>[2x]MGRIKNKQFAVIGLGKFGGSICKELHRMGHEVLAVDINEEKVNAYASYATHAVIANATEENELLSLGIRNFEYVIVAIGANIQASTLTTLLLKELDIPNIWVKAQNYYHHKVLEKIGADRIIHPEKDMGVKIAQSLSDENVLNYIDLSDEYSIVELLATRKLDSKSIIDLNVRAKYGCTILAIKHHGDICLSPAPEDIIREQDCLVIMGHKKDIKRFENEGM

KtrAB is a cation channel with a nucleotide-dependent RCK domain. The structure of the KtrAB complex revealed a homodimeric membrane protein (KtrB) assembled with a cytosolic RCK octameric ring, formed by the KtrA protein. KtrA binds nucleotides, ATP or ADP. ATP binding induces the adoption of a square-conformation by the octameric ring and increased K+ flux activity through KtrAB; ADP binding results in a non-square conformation and decreased flux.

The structures of R16K (at 2.7 Å resolution) and R16A (at 3.4 Å resolution) with ATP are very similar to that of the previously determined wild-type KtrA-ATP (WT-ATP), adopting the square conformation. In the ATP-bound rings, these distances are similar in the R16K (30.8/30.8 Å), R16A (29.9/29.9 Å) mutants and wild-type (30.0/30.0 Å) structures. A clue for the role of E125 is revealed by the 2.7 Å structure of the ATP-bound R16K KtrA mutant. In this structure, there was a distinct additional electron-density in the KtrA intra-dimer interface, between the γ-phosphates of the nucleotide. After careful crystallographic refinement, we concluded that the density likely corresponds to a magnesium ion. The ion is coordinated by six oxygen atoms, adopting octahedral geometry. The coordinating atoms are provided by the γ-phosphate of both ATP molecules, by two water molecules and by the carboxylic groups of the two E125 residues. In this structure, the K16 side-chain is well defined in the electron density, interacting with one of the Mg2+ coordinating water molecules, with the carbonyl group of Q105 from the opposite subunit and with the γ-phosphate from the ATP in the same subunit. The octahedral coordination of the ion along with the majority of the coordination distances fit well with the expected coordination of a magnesium ion; however, the interaction distances with the oxygen atoms in the phosphate groups are longer than expected. Overall, we conclude that the ion bound to the intra-dimer interface site is a magnesium ion.(2R)-2-benzyl-5-hydroxy-4-oxopentanoic 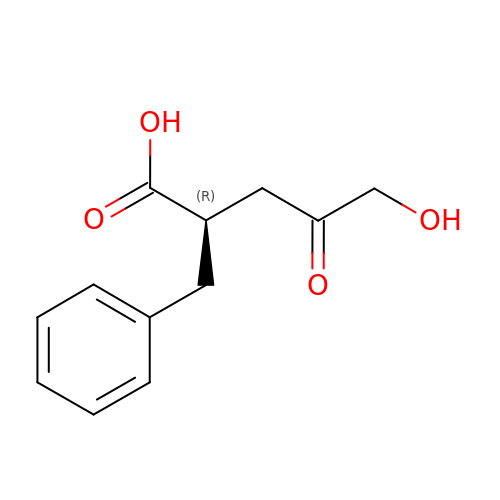acid | C12 H14 O4 | HHXVRTWUQBYAFG-SNVBAGLBSA-N N-{(3-endo)-8-[(trans-4-aminocyclohexyl)sulfonyl]-8-azabicyclo[3.2.1]octan-3-yl}-5-cyclopropyl-1,2-oxazole-3-carboxamide 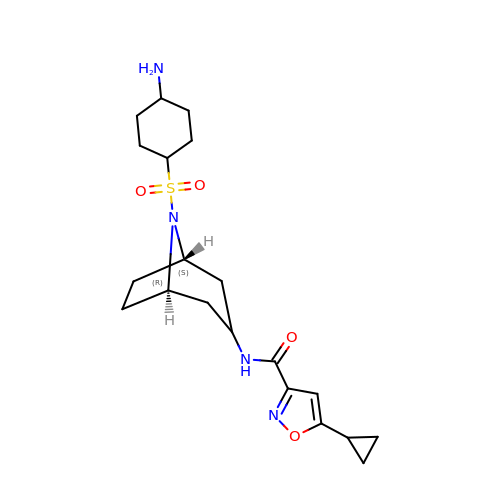| C20 H30 N4 O4 S | JYZQPJRVTADXNE-BSBCAUIJSA-N>[4x]GSHMSINIRDPLIVSRVVGDVLDPFNRSITLKVTYGQREVTNGLNLRPSQVQNKPRVEIGGEDLRNFYTLVMVDPDVPSPS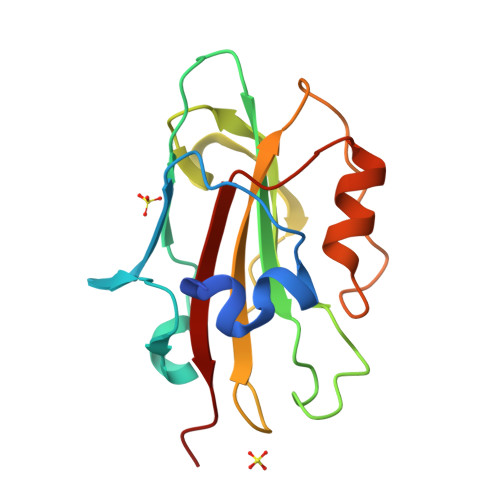NPHLREYLHWLVTDIPATTGTTFGNEIVSYENPSPTAGIHRVVFILFRQLGRQTVYAPGWRQNFNTREFAEIYNLGLPVAAVFYNSQRES1-(beta-D-ribofuranosyl)-1H-1,2,4-triazole-3-carboxamide | C8 H12 N4 O5 | 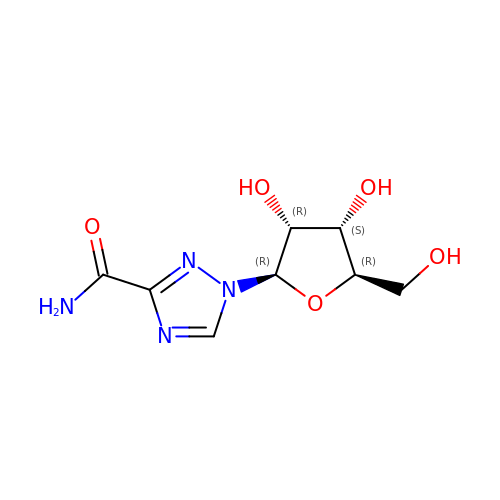IWUCXVSUMQZMFG-AFCXAGJDSA-N> DCPSDWSSYEGHCYKPFSEPKNWADAENFCTQQHAGGHLVSFQSSEEADFVVKLAFQTFGHSIFWMGLSNV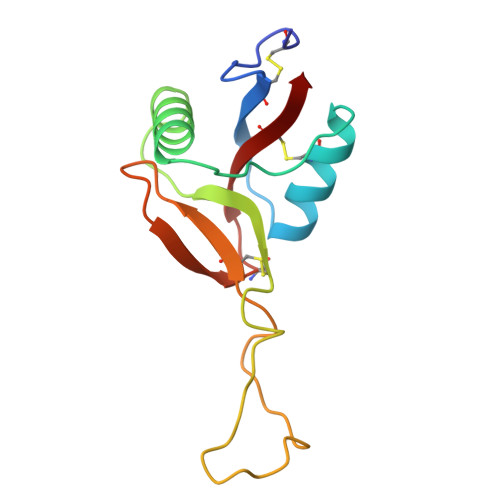WNQCNWQWSNAAMLRYKAWAEESYCVYFKSTNNKWRSRACRMMAQFVCEFQA> SAPSPQSPETPAPQNQTSRVVQAPKEEEEDEQEASEEKASEEEKAWLMASRQQLAKETSNFGFSLLRKISMRHDGNMVFSPFGMSLAMTGLMLGATGPTETQIKRGLHLQALKPTKPGLLPSLFKGLRETLSRNLELGLTQGSFAFIHKDFDVKETFFNLSKRYFDTECVPMNFRNASQAKRLMNHYINKETRGK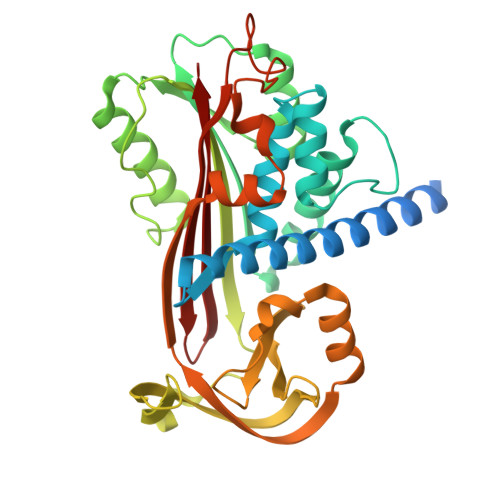IPKLFDEINPETKLILVDYILFKGKWLTPFDPVFTEVDTFHLDKYKTIKVPMMYGAGKFASTFDKNFRCHVLKLPYQGNATMLVVLMEKMGDHLALEDYLTTDLVETWLRNMKTRNMEVFFPKFKLDQKYEMHELLRQMGIRRIFSPFADLSELSATGRNLQVSRVLQRTVIEVDERGTEAVAGILSEITAR> MRTSLPSPMFSRNDFSIWSILRKCIGMELSKITMPVIFNEPLSFLQRLTEYMEHTYLIHKASSLSDPVERMQCVAAFAVSAVASQWERTGKPFNPLLGETYELVRDDLGFRLISEQVSHHPPISAFHAEGLNNDFIFHGSIYPKLKFWGKSVEAEPKGTITLELLEHNEAYTWTNPTCCVHNIIVGKLWIEQYGNVEIINHKTGDKCVLNFKPCGLFGKELHKVEGYIQDKSKKKLCALYGKWTECLYSVDPATFDAYKKNDKKNTEEKKNSKQMSTSEELDEMPVPDSESVFIIPGSVLLWRIAPRPPNSAQMYNFTSFAMVLNEVDKDMESVIPKTDCRLRPDIRAMENGEIDQASEEKKRLEEKQRAARKNRSKSEEDWKTRWFHQGPNPYNGAQDWIYSGSYWDRNYF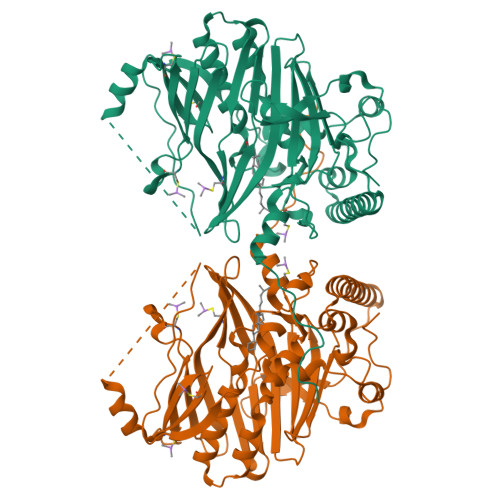NLPDIYLEHHHHHH>[7x]QAQLCDQY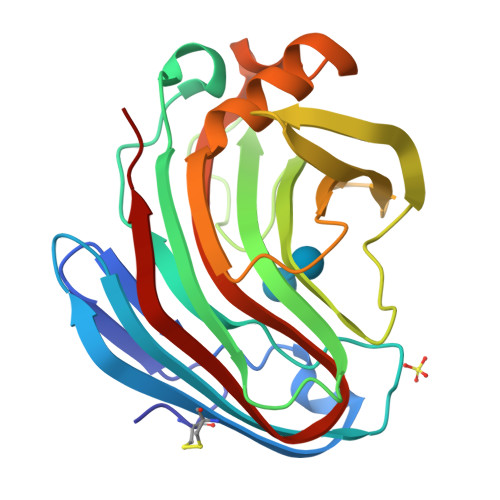ATYTGGVYTINNNLWGKDAGSGSQCTTVNSASSAGTSWSTKWNWSGGENSVKSYANSGLTFNKKLVSQISQIPTTARWSYDNTGIRADVAYDLFTAADINHVTWSGDYELMIWLARYGGVQPIGSQIATATVDGQTWELWYGANGSQKTYSFVAPTPITSFQGDVNDFFKYLTQNHGFPASSQYLITLQFGTAPFTGGPATLSVSNWSASVQ> NRFYLLTLTSNKDESITLAIDVEDMVAVAYQPAGSHESYFFLNAPQLAFHTLFTDTHQNVLNFDNTFKSLENAAGTTRQTIVLGVDPLDFAISNLFNADPKLLPLSFLVIIQMVLEASKFRFIEQSVAYSFKNEKTFIPDLAIVSLEDNWSEISLQIQASTSLQGLFGSVVELYNSNNELIEVDSIYYPIILANVALQLYHCQVS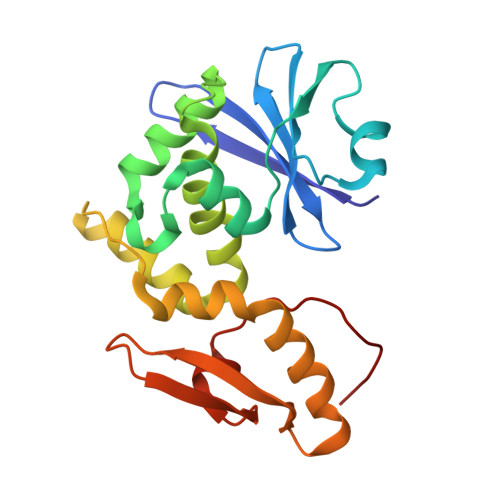T>MKGTIVGTWIKTLRDLYGNDVVDESLKSVGWEPDRVITPLEDIDDDEVRRIFAKVSEKTGKNVNEIWREVGRQNIKTFSEWFPSYFAGRRLVNFLMMMDEVHLQL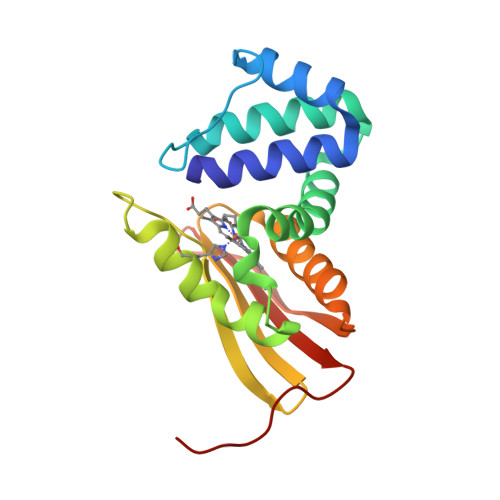TKMIKGATPPRLIAKPVAKDAIEMEYVSKRKMYDYFLGLIEGSSKFFKEEISVEEVERGEKDGFSRLKVRIKFKNPVFEYKKN[2x]> MDIVFAADDNYAAYLCVAAKSVEAAHPDTEIRFHVLDAGISEANRAAVAANLRGGGGNIRFIDVNPEDFAGFPLNIRHISITTYARLKLGEYIADCDKVLYLDIDVLVRDSLTPLWDTDLGDNWLGASIDLFVERQEGYKQKIGMADGEYYFNAGVLLINLKKWRRHDIFKMSSEWVEQYKDVMQYQDQDILNGLFKGGVCYANSRFNFMPTNYAFMANWFASRHTDPLYRDRTNTVMPVAVSHYCGPAKPWHRDCTAWGAERFTEL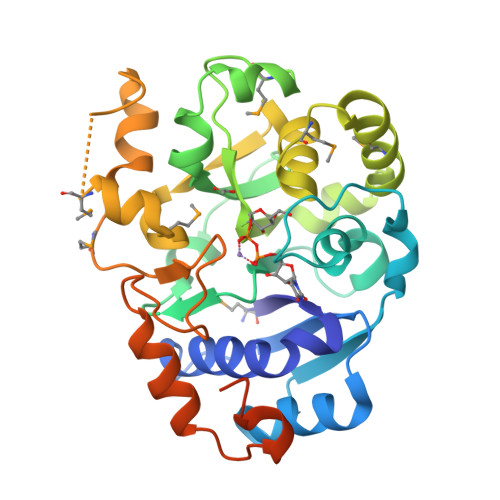AGSLTTVPEEWRGKLAVPHRMFSTKRMLQRWRRKLSARFLRKIY(2~{R})-2-azanyl-~{N}-(4-oxidanylidene-6,7-dihydro-5~{H}-1,3-benzothiazol-2-yl)propanamide | C10 H13 N3 O2 S | 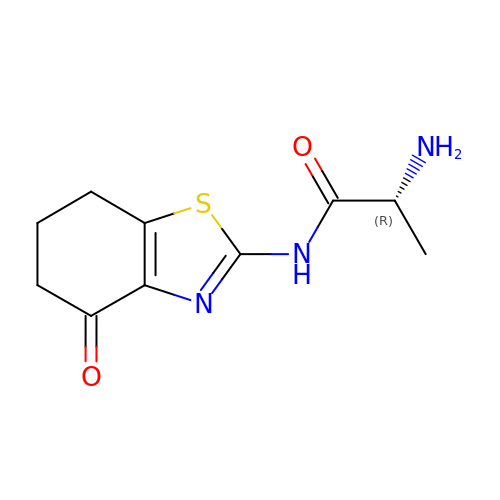IOUBCOWUBQDGKF-RXMQYKEDSA-N>[2x]RTVSSLKNLLSENLTLIKEKTGNSSDIVIRHFKIGVNNSLAAAIVYIEGIVDNQAIQDYLLQSLMKDNQKNDLNDQNALELISEDIVTMGNVSFADNWNDLLSSLMSGDSLLIVDGINRVLSVSTQGGEKRAIAESTTQMVVRGPKGAFTESIGTNLAMVRRIIKTPDLWLES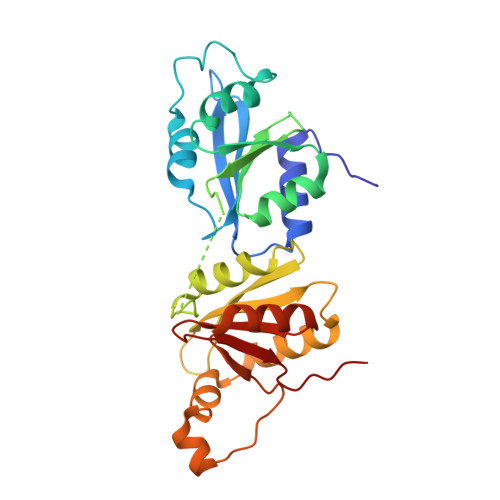MKIGRVTKTDVTLMYIHGIANDKVVKEIRKRLKNIDIDSILESGYVEQLIEDQTVTPFPTIYNTERPDVVAGNLLEGRIAIFVDGTPFGLIAPALFIQF>MKTTSFILALIISISIGKAQTNHQVSYFSLQDVKLLSSPFLQAQQTDLHYILALDPDRLSAPFLREAGLTPKAPSYTNWENTGLDGHIGGHYLSALSMMYAATGDTAIYHRLNYMLNELHRAQQAVGTGFIGGTPGSLQLWKEIKAGDIRAGGFSLNGKWVPLYNIHKTYAGLRDAYLYAHSDLARQMLIDLTDWMIDITSGLSDNQMQDMLRSEHGGLNETFADVAEITGDKKYLKLARRFSHKVILDPLIKNEDRLNGMHANTQIPKVIGYKRVAEVSKNDKDWNHAAEWDHAARFFWNTVVNHRSVCIGGNSVREHFHPSDNFTSMLNDVQGPETCNTYNMLRLTKMLYQNSGDVDNSNKPDPRYVDYYERALYNHILSSQEPDKGGFVYFTPMRPGHYRVYSQPETSMWCCVGSGLENHTKYGEFIYAHQQDTLYVNLFIPSQLNWKEQGVTLTQETLFPDDEKVTLRIDKAAKKNLTLMIRIPEWAGNSKGYEITINGKKHLSDIQTGASTYLPIRRKWKKGDMITFHLPMKVSLEQIPDKKDYYAFLYGPIVLATSTGTENLDGIYADDSRGGHIAHGRQTPLQEIPMLIGNPDSIRHSLHKLSGSKLAFSYDGNVYPTQKSKSLELIPFFRLHNSRYAVYFRQASEEQFKTIQEEMATAERKATELANRTVDLIFPGEQQPESDHSIQYEASETGTHKDRHFRRAKGWFSYNLKIKEEASQLMITVRQEDRNKAVILLNNEKLTVHPTVSKADKDGFIRLCYLLPRKLKVGSCEILFKPDGTEWTSAVYEVRLLK[2x]

pmcβ-l-Arabinofuranosidases hydrolyze β-l-arabinofuranosyl units from arabino-oligosaccharides (AOS), complex pectic dietary glycans, and plant-derived glycoproteins such as solanaceous lectins. Two representative examples of gut microbiome β-l-arabinofuranosidases and the subject of the herein-presented studies are HypBA1 (classified within GH127 and expressed by B. longum) and BtGH146 (GH146, expressed by B. thetaiotaomicron). We recently reported that both Bacteroides thetaiotaomicronBtGH146 and Bifidobacterium longum HypBA1 are inhibited by β-l-arabinofuranosyl cyclophellitol epoxide, supporting the action of a zinc-coordinated cysteine as a catalytic nucleophile, where in most retaining GH families, an aspartate or glutamate is employed. The β-l-arabinofuranosyl cyclophellitol aziridines both inhibit and label β-l-arabinofuranosidase efficiently (however with different activities), whereas the epoxide-derived probes favor BtGH146 over HypBA1. These findings are accompanied by X-ray structural analysis of the unmodified β-l-arabinofuranosyl cyclophellitol aziridine in complex with both isozymes, which were shown to react by nucleophilic opening of the aziridine, at the pseudoanomeric carbon, by the active site cysteine nucleophile to form a stable thioether bond.

In order to gain structural insights into the reactivity of aziridine 2 with rHypBA1 and rBtGH146, it was cocrystallized with both enzymes, and the resulting complexes were studied by X-ray diffraction. Electron density for the carbon emulating the anomeric center (C1) in aziridine 2 was observed at covalent bond distance from the catalytic nucleophile residue in both isozymes (C416 for rBtGH146 in Figure 3A; C417 for rHypBA1 in Figure 3B). The covalent complex of rBtGH146 with aziridine 2 displayed the anomeric-mimicking carbon C1 at covalent bond distance to the thiol group of C416. This points to the expected regiochemical outcome as for conventional retaining glycosidases30−34 and provides further evidence supporting annotation of this enzyme, like rHypBA1, as a retaining β-l-arabinofuranosidase utilizing a cysteine catalytic site nucleophile. In particular, the primary hydroxyl O5 in 2 was involved in H-bond interactions with distinct H-bond acceptor residues within the binding pocket—these are E217 in rBtGH146:2 and H142 in rHypBA1:2. However, no cysteine equivalent to C415 of rHypBA1 is present in the active site of rBtGH146. In the rBtGH146:2 complex, N1 of 2 interacts exclusively with a proximal glutamine (Q689) in the active site. The crystal structure of 1 in complex with BtGH146 revealed an unexpected regiochemical reactivity: the catalytic nucleophile C416 appeared to have formed a covalent bond with the pseudoanomeric carbon (that is, C6 in 1), instead of the expected carbon17−21 corresponding to the anomeric center of the parent substrate (C1 in 1), while the HypBA1 catalytic nucleophilic cysteine reacted at the carbon mimicking the anomeric center (C1).>SVLQVLHIPDERLRKVAKPVEEVNAEIQRIVDDMFETMYAEEGIGLAATQVDIHQR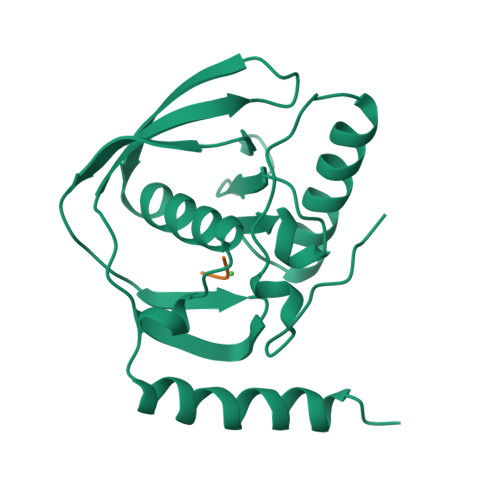IIVIDVSENRDERLVLINPELLEKSGETGIEEGCLSIPEQRALVPRAEKVKIRALDRDGKPFELEADGLLAICIQHEMDHLVGKLFMDYLSPLKQQRIRQKVEKLDRLKARA[3x];>[3x]MAS>MLKGKVALVTGASRGIGRAIAIDLAKQGANVVVNYAGNEQKANEVVDEIKKLGSDAIAVRADVANAEDVTNMVKQTVDVFGQVDILVNNAGVTKDNLLMRMKEEEWDTVINTNLKGVFLCTKAVSRFMMRQRHGRIVNIASVVGVTGNPGQANYVAAKAGVIGLTKTSAKELASRNITVNAIAPGFIATDMTDVLDENIKAEMLKLIPAAQFGEAQDIANAVTFFASDQSKYITGQTLNVDG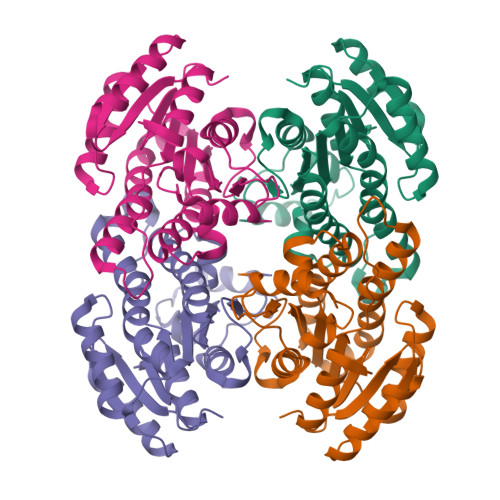GMVM[8x]4-[(2S)-2-amino-3-hydroxypropyl]phenol 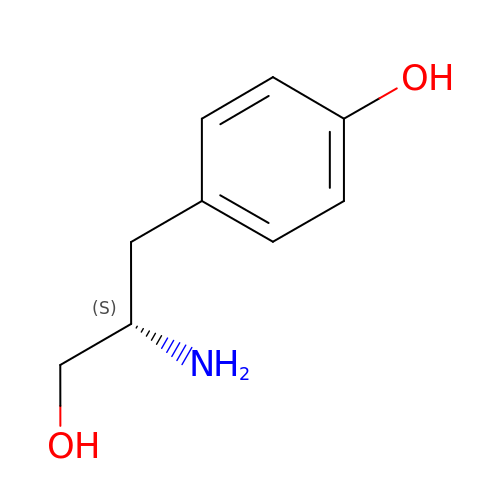| C9 H13 N O2 | DBLDQZASZZMNSL-QMMMGPOBSA-N5-[3-(1~{H}-indol-3-yl)propoxy]-1-phenyl-pyrazole-4-carboxylic acid | C21 H19 N3 O3 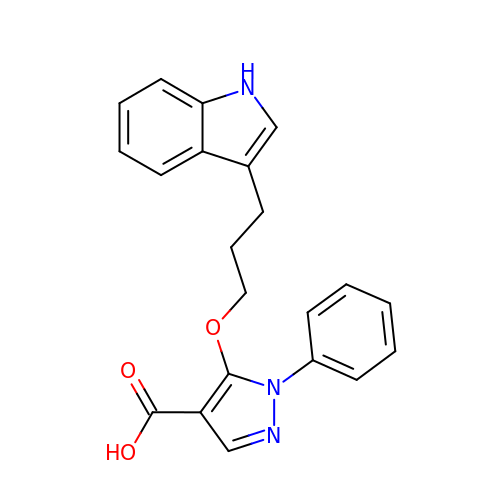| KHUCHDHRSOJGSA-UHFFFAOYSA-N>MSYYHHHHHHLESTSLYKKAGSMAVDADSANYRIEHDTMGEVRVPAKALWRAQTQRAVENFPISGRGLERTQIRALGLLKGACAQVNSDLGLLAPEKADAIIAAAAEIADGQHDDQFPIDVFQTGSGTSSNMNTNEVIASIAAKGGVTLHPNDDVNMSQSSNDTFPTATHIAATEAAVAHLIPALQQLHDALAAKALDWHTVVKSGRTHLMDAVPVTLGQEFSGYARQIEAGIERVRACLPRLGELAIGGTAVGTGLNAPDDFGVRVVAVLVAQTGL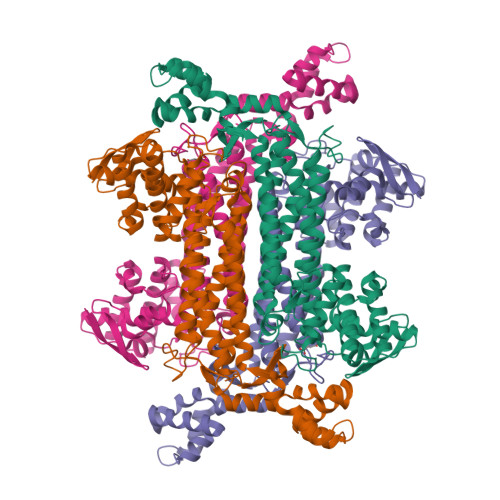SELRTAANSFEAQAARDGLVEASGALRTIAVSLTKIANDIRWMGSGPLTGLAEIQLPDLQPGSSIMPGKVNPVLPEAVTQVAAQVIGNDAAIAWGGANGAFELNVYIPMMARNILESFKLLTNVSRLFAQRCIAGLTANVEHLRRLAESSPSIVTPLNSAIGYEEAAAVAKQALKERKTIRQTVIDRGLIGDRLSIEDLDRRLDVLAMAKAEQLDSDR[4x]>[2x]MGHHHHHHHHHHSSGHIEGRHMAAHQLSDFQRNKILRVFNTFYDCNHDGVIEWDDFELAIKKICNLHS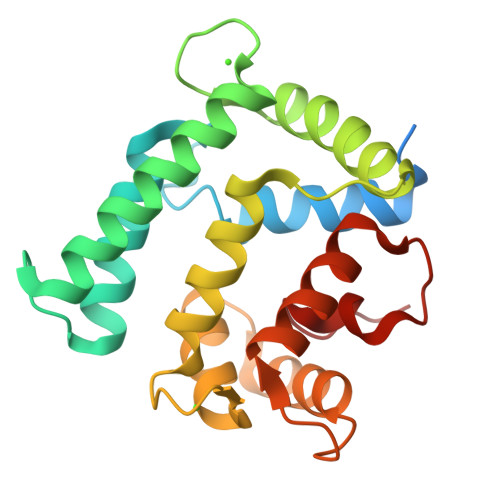WPTDGKKHNEARATLKLIWDGLRKYADENEDEQVTKEEWLKMWAECVKSVEKGESLPEWLTKYMNFMFDVNDTSGDNIIDKHEYSTVYMSYGIPKSDCDAAFDTLSDGGKTMVTREIFARLWTEYFVSNDRGAKGNHLFGDLKL> A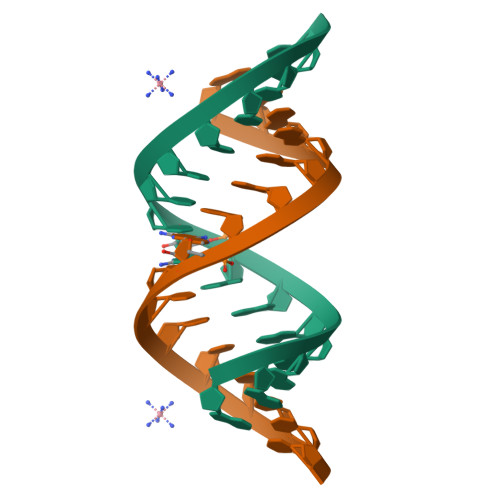GAGAAGGUCUUCUCU> MAFEALTGINGDLITRSWSASKQAYLTERYHKEEAGAVVIFAFQPSFSEKDFFDPDNKSSFGEIKLNRVQFPCMRKIGKGDVATVNEAFLKNLEAIIDPRTSFQASVEMAVRSRKQIVFTGHSSGGATAILATVWYLEKYFIRNPNVYLEPRCVTFGAPLVGDSIFSHALGREKWSRFFVNFVSRFDIVPRIMLARKASVEETLPHVLAQLDPRKSSVQESEQRITEFYTRVMRDTSTVANQAVCELTGSAEAFLETLSSFLELSPYRPAGTFVFSTEKRLVAVNNSDAILQMLFYTSQASDEQEWSLIPFRSIRDHHSYEELVQSMGKKLFNHLDGENSIESTLNDLGVSTRGRQYVQAALEEEKKRVENQKKIIQVIEQERFLKKLAWIEDEYKPKCQAHKNGYYDSFKVSNEENDFKANVKRAELAGVFDEVLGLMKKCQLPDEFEGDIDWIKLATRYRRLVEPLDIANYHRHLKNEDTGPYMKRGRPTRYIYAQRGYEHYILKPNGMIAEDVFWNKVNGLNLGLQLEEIQETLKNSGSECGSCFWAEVEELKGKPYEEVEVRVKTLEGMLGEWI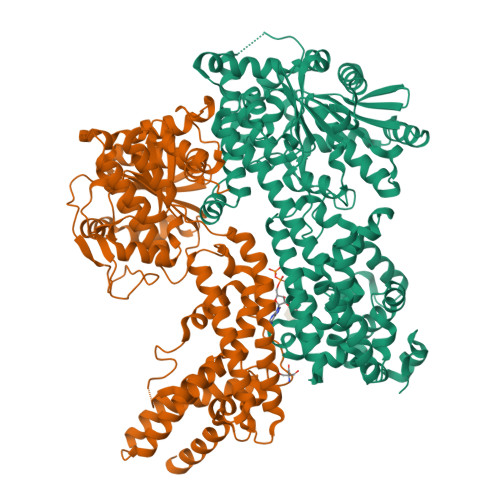TDGEVDDKEIFLEGSTFRKWWITLPKNHKSHSPLRDYMMDEITDT;> MDDCRFETSELQASVMISTPLFTDSWSSCNTANCNGSIKIHDIAGITYVAIPAVSMIQLGNLVGLPVTGDVLFPGLSSDEPLPMVDAAILKLFLQLKIKEGLELELLGKKLVVITGHSTGGALAAFTALWLLSQSSPPSFRVFCITFGSPLLGNQSLSTSISRSRLAHNFCHVVSIHDLVPRSSNEQFWPFGTYLFCSDKGGVCLDNAGSVRLMFNILNTTATQNTEEHQRYGHYVFTLSHMFLKSRSFLGGSIPDNSYQAGVALAVEALGFSNDDTSGVLVKECIETATRIVRAPILRSAELANELASVLPARLEIQWYKDRCDASEEQLGYYDFFKRYSLKRDFKVNMSRIRLAKFWDTVIKMVETNELPFDFHLGKKWIYASQFYQLLAEPLDIANFYKNRDIKTGGHYLEGNRPKRYEVIDKWQKGVKVPEECVRSRYASTTQDTCFWAKLEQAKEWLDEARKESSDPQRRSLLREKIVPFESYANTLVTKKEVSLDVKAKNSSYSVWEANLKEFKCKMGYENEIEMVVDESDAMET> SSMRKIC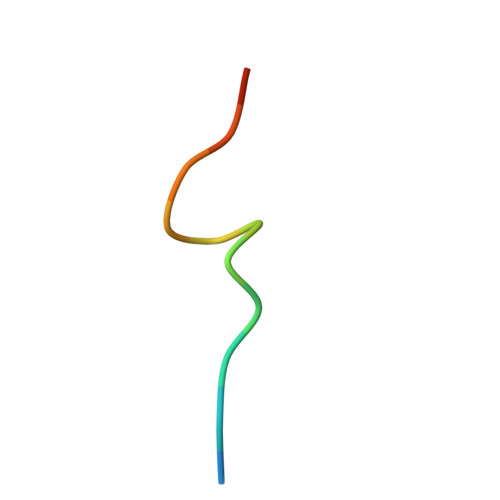TYFHRKS>ADKELKFLVVDDFSTMRRIVRN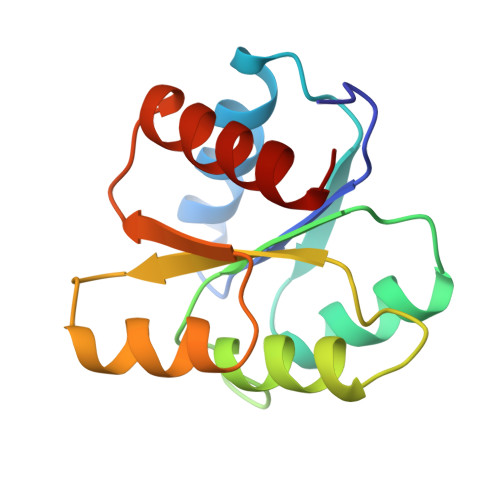LLKELGFNNVEEAEDGVDALNKLQAGGYGFVISDWNMPNMDGLELLKTIRADGAMSALPVLMVIAEAKKENIIAAAQAGASGWVVKPFTAATLEEKLNKIFEKLGM[2x]>MQITLARIDDRLIHGQVTTVWSKVANAQRIIICNDDVFNDEVRRTLLRQAAPPGMKVNVVSLEKAVAVYHNPQYQDETVFYLFTNPHDVLTMVRQGVQIATLNIGGMAWRPGKKQLTKAVSLDPQDIQAFRELDKLGVKLDLRVVASDPSVNILDKINE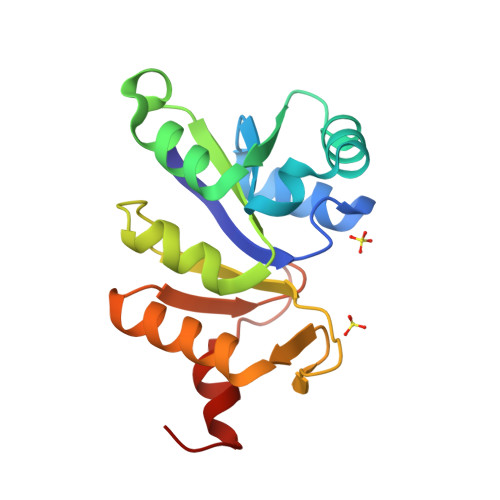TAFCE[4x]Cellular compartments maintain a reducing environment by constant recycling of oxidized antioxidants back to their reduced forms, a reaction catalyzed by glutathione reductase (GR) in the case of oxidized glutathione (GSSG) and dehydroascorbate reductase (DHAR) for dehydroascorbate (DHA), the oxidized form of AsA11. Whereas GSH is relatively stable in its oxidized form, DHA undergoes irreversible hydrolysis to diketogluonate (DKG), and therefore, rapid reduction of DHA in cells is critical for effective AsA recycling. Previously, DHAR has been reported to have a bi-uni-uni-uni ping-pong enzymatic mechanism, with GSH and DHA interacting with the catalytic cysteine (Cys20 in AtDHAR2) in separate, sequential binding events. AtDHAR2 crystallized as a monomer and exhibited the classic structural architecture common to the GST super-family, with an all-helical C-terminal domain, and a thioredoxin-like N-terminal domain consisting of a mixture of β-sheets and α-helices.

The crystal structure of AtDHAR2 in complex with GSH was solved by molecular replacement to a resolution of 2.3 Å in space group P21221. GSH was placed into the available electron density of the mFO-DFC difference map at the G-site of AtDHAR2 at full occupancy in a non-covalently bound state. The cysteinyl sulfur of GSH was in close proximity (2.8 Å) to the sulfur atom of Cys20, thereby indicating that the GSH was likely engaged in a mixed disulfide (for which a maximum bond length of 2.3 Å is commonly applied) with Cys20 before disulfide cleavage by X-ray irradiation, a well-characterized phenomenon. The GSH γ-glutamyl is particularly well stabilized, as evidenced by low B-factor values of 24–29 Å2, accepts H-bonds to its carboxylate from a water molecule and from the backbone amide and side-chain hydroxyl of Ser73, and forms a salt bridge interaction with Asp72 via its amine group. The central cysteinyl region of the GSH molecule is stabilized by hydrogen bonding of the carbonyl and amide of the cysteine with the backbone amide and carbonyl groups of Val60. The glycinyl group of GSH is less tightly bound, as reflected by elevated B-factors of 39–48 Å2, forming a single salt bridge with the side-chain amine of Lys47 through its carboxylate. The overall structural fold of AtDHAR2 is almost identical to that of the structures of OsDHAR1 and PgDHAR1, albeit with the inclusion of an additional short-chain helical turn preceding the α1-helix. The introduction of the α1’-helix in AtDHAR2 alters the peptide torsion of Asp19 in such a way as to re-direct its side-chain carboxylate toward the protein interior, forming a hydrogen bond with His160. However, although Lys8 is conserved in AtDHAR2, it is instead positioned at the beginning of the β1-strand, distal from the active site cleft and 19 Å Cα-Cα from the positioning of Lys8 of OsDHAR1, and the equivalent position occupied by a glycine.

> GPMALDICVKVAVGAPDVLGDCPFSQRVLLTLEEKKLPYKTHLINVSDKPQWFLDISPEGKVPVVKLDGKWVADSDVIVGLLEEKYPEPSLKTPPEFASVGSKIFGAFVTFLKSKDANDGSEKALVDELEALENHLKTHSGPFVAGEKITAVDLSLAPKLYHLEVALGHYKNWSVPESLTSVRNYAKALFSRESFENTKAKKEIVVAGWESKVNA> MPKHGKRYRALLEKVDPNKIYTIDEAAHLVKELATAKFDETVEVHAKLGIDPRRSDQNVRGTVSLPHGLGKQVRVLAIAKGEKIKEAEEAGADYVGGEEIIQKILDGWMDFDAVVATPDVMGAVGSKLGRILGPRGLLPNPKAGTVGFNIGEIIREIKAGRIEFRNDKTGAIHAPVGKASFPPEKLA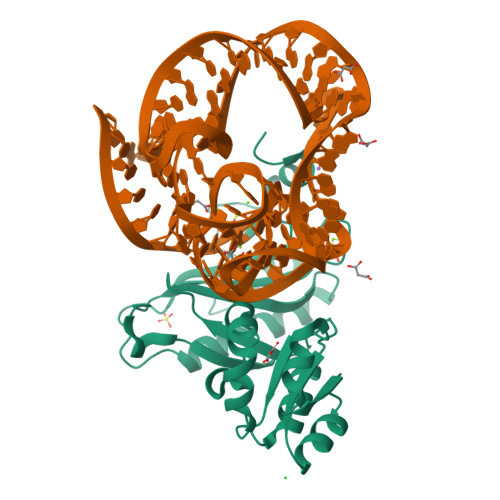DNIRAFIRALEAHKPEGAKGTFLRSVYVTTTMGPSVRINPHS> APDSVDYRKKGYVTPVKNQGQCGSCWAFSSVGALEGQLKKKTGKLLNLSPQNLVDCVSENDGCGGGYMTNAFQYVQKNRGIDSEDAYPYVGQEESCMYNPTGKAAKCRGYREIPEGNEKALKRAVARVGPVSVAIDASLTSFQFYSKGVYYDESCNSDNLNHAVLAVGYGIQKGNKHWIIKNSWGENWGNKGYILMARNKNNACGIANLASFPKM

Cathepsin K (CatK) is one of the most investigated cysteine cathepsins, both by academia and pharmaceutical companies. It is expressed in high levels in osteoclasts, where it serves as the principal protease involved in bone remodelling. Cathepsin K (CatK) is a target for the treatment of osteoporosis, arthritis, and bone metastasis. Peptidomimetics with a cyanohydrazide warhead represent a new class of highly potent CatK inhibitors; however, their binding mechanism is unknown.

The cyanohydrazide warhead positioned centrally in the inhibitor molecule forms a covalent isothiosemicarbazide adduct with a thiol group of the catalytic Cys25. The nitrogen atom of the imidate moiety of Gü2602 is strongly stabilised by three hydrogen bonds to the backbone amide of the catalytic Cys25, carbonyl group of Gly23, and the side chain amide of Gln19. In contrast to Gü1303, there is no hydrogen bonding between Gü2602 and the Gly66 residue. However, a new hydrogen bond is formed between the backbone oxygen of Asn161 and the amide NH of Gü2602. The P2 Boc-capping group resides in the S2 subsite of mCatK and makes nonpolar interactions with Tyr67, Leu160, and Ala163. The B-factor values were generally in the low range, but increased values were only found for the P1 N-benzyl-N-methylacetamide part of Gü2602, with the highest value for its benzyl group. An analogous B-factor pattern was also observed for inhibitors in iCatK complexes. This finding indicated an increased flexibility and dynamic disorder of the major crystallographic conformation of the benzyl group of Gü2602, which is located in the non-primed part of the active site and oriented out of the S1 subsite. In contrast, Gü2602 primarily occupies the S2 subsite, and the N-benzyl-N-methylacetamide part (especially its benzyl moiety) is highly flexible and has two alternative types of conformations that reside in the non-primed part (the S1 subsite) or primed part (the S2’ subsite) of the active site. We hypothesise that the conformational flexibility of the complexed ligand at the boundary of the non-primed and primed subsites provides an entropic advantage contributing to the extraordinary potency of Gü2602 in the low picomolar range.>[4x]STYNGPLSSHWFPEELAQWEPDSDPDAPFNRSHVPLEPGRVADRVNANADKDAHLVSLSALNRHTSGVPSQGAPVFYENTFSYWHYTDLMVYWAGSAGEGIIVPPSADVIDASHRNGVPILGNVFFPPTVYGGQLEWLEQMLEQEEDGSFPLADKLLEVADYYGFDGWFINQETEGADEGTAEAMQAFLVYLQEQKPEGMHIMWYDSMIDTGAIAWQNHLTDRNKMYLQNGSTRVADSMFLNFWWRDQRQSNELAQALGRSPYDLYAGVDVEARGTSTPVQWEGLFPEGEKAHTSLGLYRPDWAFQSSETMEAFYEKELQFWVGSTGNPAETDGQSNWPGMAHWFPAKSTATSVPFVTHFNTGSGAQFSAEGKTVSEQEWNNRSLQDVLPTWRWIQHGGDLEATFSWEEAFEG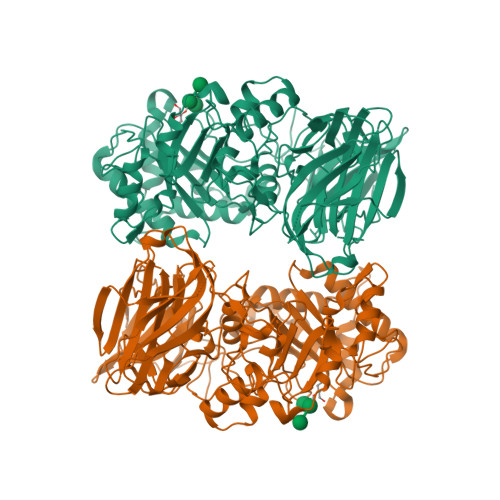GSSLQWHGSLAEGEHAQIELYQTELPISEGTSLTWTFKSEHDNDLNVGFRLDGEEDFRYVEGEQRESINGWTQWTLPLDAFAGQTITGLAFAAEGNETGLAEFYTGQLAVGADSEKPAAPNVNVRQYDPDPSGIQLVWEKQSNVHHYRVYKETKHGKELIGTSAGDRIYIEGLVEESKQNDVRLHIEALSETFVPSDARMIDIKSGSF>SNVPHKSSLPEGIRPGTVLRIRGLVPPNASRFHVNLLCGEEQGSDAALHFNPRLDTSEVVFNSKEQGSWGREERGPGVPFQRGQPFE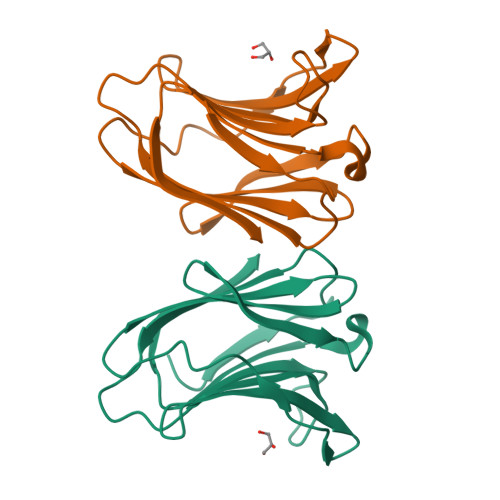VLIIASADGFKAVVGDAQYHHFRHRLPLARVRLVEVGGDVQLDSVRIF[2x]> GAMDKQKPRYEIRWRVIESISPDGHEYIYVDPMQLPYDSRWEFPRDGLVL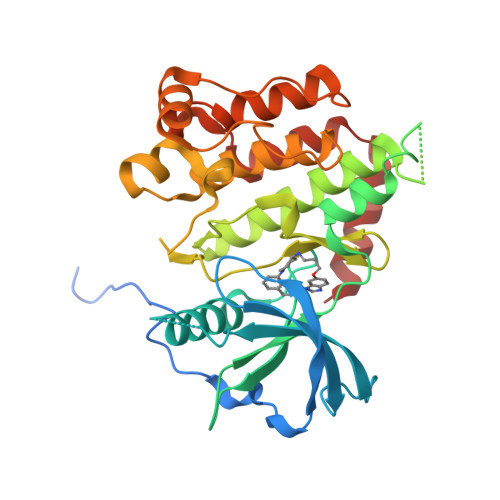GRVLGSGAFGKVVEGTAYGLSRSQPVMKVAVKMLKPTARSSSKQALMSELKIMTHLGPHLNIVNLLGACTKSGPIYIIIEYCFYGDLVNYLHKNRDSFLSHKKKSMLDSEVKNLLSDDNSEGLTLLDLLSFTYQVARGMEFLASKNCVHRDLAARNVLLAQGKIVKICDFGLARDIMHDSNYVSKGSTFLPVKWMAPESIFDNLYTTLSDVWSYGILLWEIFSLGGTPYPGMMVDSTFYNKIKSGYRMAKPDHATSEVYEIMVKCWNSEPEKRPSFYHLSEIVENLLPGQYKKSYEKIHLDFLKSD>[2x]MASSN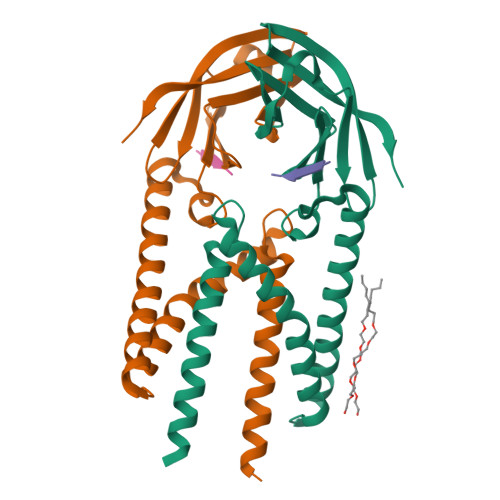VTLSNDEVLRLVKDWNFTWSVVFLLITIVLQYGYPSRSMFVYVIKMFVLWLLWPASMALSIFCAVYPIDLASQIISGILAATSCAMWISYFVQSIRLFMRTGSWWSFNPESNCLLNVPIGGTTVVRPLVEDSTSVTAVVTDGYLKMAGMHFGACDFQRLPSEVTVAKPNVLIALKMIKRQAYGTNSGVAIYHRYKAGNYRRPPIIQDQELALLRA;>AAAAA[2x]>[2x]GPHMETETSFFDLYDVDLKDKRSVIGKGAFSTVHRCVNKRTGEVCA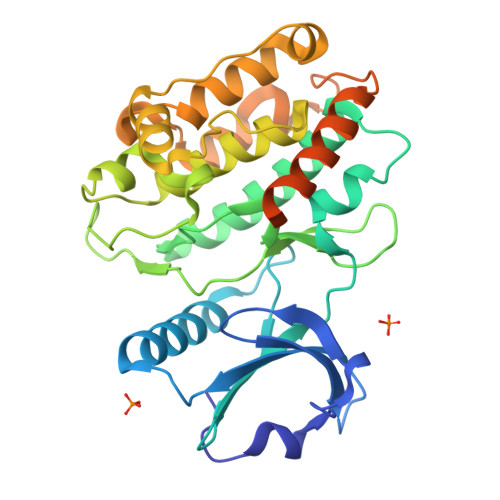VKVIALKSLRSSEINKIKREIGICSSLQHEHIVSMRRAFRDESHFYLVFEYVSGGELFDEIVTRKFYNEKDASACMHQILSALQHCHSKNIIHRDLKPENLLLASKDPNAPVKITDFGLAVIMEQGPTYFGFAGTPGYLSPEVIRRVPYDTAVDVWACGVILYILLVGYPPFWEEDHQKLYAQIKNCQYDFPSPEWDSVTTAAKELIKAMLEPNPKRRPTVQELLQHPWIARRDVPGSVHRQATLEELKKFNARRKLKGGVNAVIGVSKMMRTMQEATRALTLSAKSAAALEHHHHHH> MILDTDYITEDGKPVIRIFKKENGEFKIEYDRTFEPYFYALLKDDSAIEEVKKITAERHGTVVTVKRVEKVQKKFLGRPVEVWKLYFTHPQDVPAIRDKIREHPAVIDIYEYDIPFAKRYLIDKGLVPMEGDEELKMLAFDIETLYHEGEEFAEGPILMISYADEEGARVITWKNVDLPYVDVVSTEREMIKRFLRVVKEKDPDVLITYNGDNFDFAYLKKRCEKLGINFALGRDGSEPKIQRMGDRFAVEVKGRIHFDLYPVIRRTINLPTYTLEAVYEAVFGQPKEKVYAEEITTAWETGENLERVARYSMEDAKVTYELGKEFLPMEAQLSRLIGQSLWDVSRSSTGNL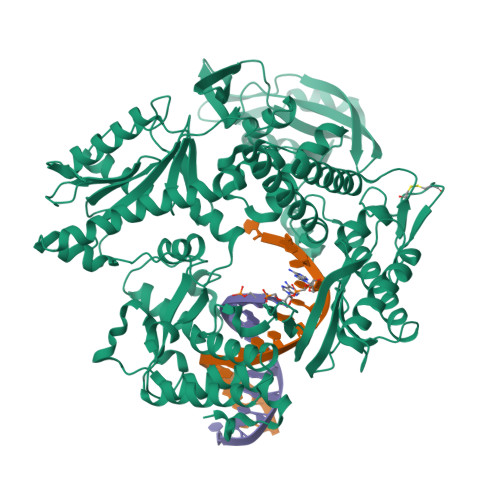VEWFLLRKAYERNELAPNKPDEKELARRRQSYEGGYVKEPERGLWENIVYLDFRSLYPSIIITHNVSPDTLNREGCKEYDVAPQVGHRFCKDFPGFIPSLLGDLLEERQKIKKKMKATIDPIERKLLDYRQRRIKILASSYYGYYGYARARWYCKECAESVTAWGREYITMTIKEIEEKYGFKVIYSDTDGFFATIPGADAETVKKKAMEFLKYINAKLPGALELEYEGFYKRGFFVTKKKYAVIDEEGKITTGGLEIVRRDWSEIAKETQARVLEALLKDGDVEKAVRIVKEVTEKLSKYEVPPEKLVIHEQITRDLKDYKATGPHVAVAKRLAARGVKIRPGTVISYIVLKGSGRIGDRAIPFDEFDPAKHKYDAEYYIENQVLPAVERILRAFGYRKEDLRYQKTRQVGLSAWLKPKGT> MGPAKQYDSVECPFCDEVSKYEKLAKIGQGTFGEVFKARHRKTGQKVALKKVLMENEKEGFPITALREIKILQLLKHENVVNLIEICRTKASPYNRCKASIYLVFDFCEHDLAGLLSNVLVKFTLSEIKRVMQMLLNGLYYIHRNKILHRDMKAANVLITRDGVLKLADFGLARAFSLAKNSQPNRYTNRVVTLWYRPPELLLGERDYGPPIDLWGAGCIMAEMWTRSPIMQGNTEQHQLALISQLCGSITPEVWPNVDNYELYEKLELVK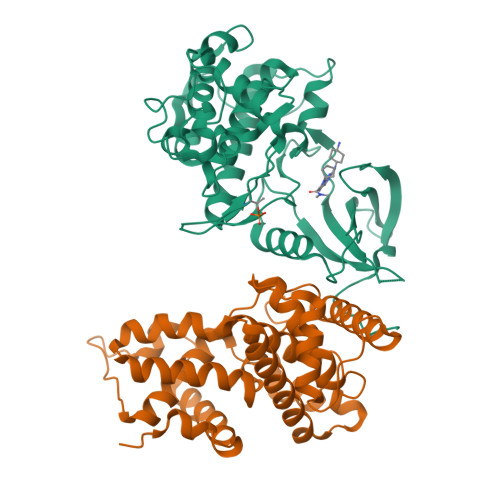GQKRKVKDRLKAYVRDPYALDLIDKLLVLDPAQRIDSDDALNHDFFWSDPMPSDLKGMLST;> PEGERKNNNKRWYFTREQLENSPSRRFGVDPDKELSYRQQAANLLQDMGQRLNVSQLTINTAIVYMHRFYMIQSFTRFPGNSVAPAALFLAAKVEGQPKKLEHVIKVAHTCLHPQESLPDTRSEAYLQQVQDLVILESIILQTLGFELTIDHPHTHVVKCTQLVRASKDLAQTSYFMATNSLHLTTFSLQYTPPVVACVCIHLACKWSNWEIPVSTDGKHWWEYVDATVTLELLDELTHELLQILEKTPNRLKRIWNWR>[2x]MESPSSEEEKPLAKMAFTLADRVTEEMLADKAALVVEVVEENYHDAPIVGIAVVNEHGRFFLRPETALADPQFVAWLGDETKKKSMFDSKRAAVALKWKGIELCGVSFDLLLAAYLLDPAQGVDDVAAAAKMKQYEAVRPDEAVYGKGAKRAVPDEPVLAEHLVRKAAAIWELERPFLDELRRNEQDRLLVELEQPLSSILAEMEFAG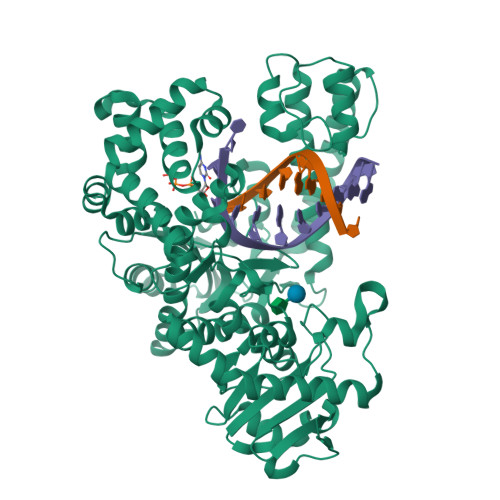VKVDTKRLEQMGKELAEQLGTVEQRIYELAGQEFNINSPKQLGVILFEKLQLPVLKKTKTGYSTSADVLEKLAPYHEIVENILHYRQLGKLQSTYIEGLLKVVRPATKKVHTIFNQALTQTGRLSSTEPNLQNIPIRLEEGRKIRQAFVPSESDWLIFAADYSQIELRVLAHIAEDDNLMEAFRRDLDIHTKTAMDIFQVSEDEVTPNMRRQAKAVNYGIVYGISDYGLAQNLNISRKEAAEFIERYFESFPGVKRYMENIVQEAKQKGYVTTLLHRRRYLPDITSRNFNVRSFAERMAMNTPIQGSAADIIKKAMIDLNARLKEERLQAHLLLQVHDELILEAPKEEMERLCRLVPEVMEQAVTLRVPLKVDYHYGSTWYDAK> MKFKAQSLTATVVFALCATASMSRAADATQDGIQRTVDAAIRPLMAKDGIHGMAVGIVAGGKAYVYNYGVASAETGKPVTRDTLFELGSISKTFTATLASYAQVSGNLSLSDTTGKYLPVLQGSQFGNVKLINLGTHTPGGLPLQVPDEIHDNDELMQYFKAWRPSCVPGACRTYTNPGIGTLGLITAKSMGEDFTPLMEQRMFPALGLKNSYIDVPEARIPDYAQGYKKDGAPIRMAPGVLSAEAYGVKSTAADMTRFMQANMNLLPLDAKLQRAIMQTHTGYFKAGVLTQDLIWEQYAYPVAL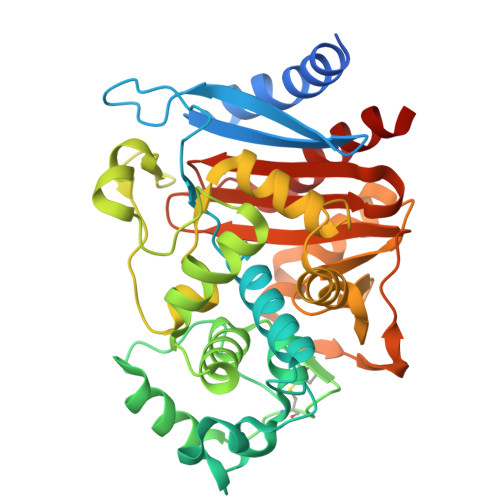KTLLAGNSSAMALKATPAVEIKPPLAPRQDVWINKTGSTNGFGAYVAFVPEKQLGIVMLANKNFPNDERVSVAYKILTALAGAGVQ> MKFTYLVSLAAFAVTALGSRPTPPNLEFLFSANLTKGPAYIYDQSDAQIKALQTLTGGIIAGPNFDGTVIGGTALSTRGADGTIRADAH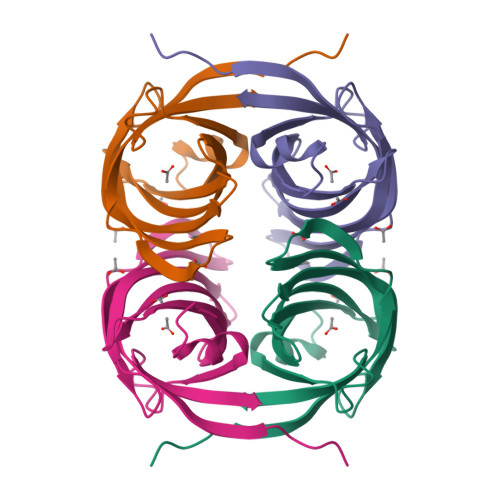YLIQTSDGANILVTESAAIPYVAVLFDTSSEKYNWLNNVTAWGTPPNLNEINFLEYWQIE>[4x]MNTIDAEVIIVGAGPTGLMLAGELRLNNVSTIVLDRLAEPMQQSRALGFSARTIEEFDQRGL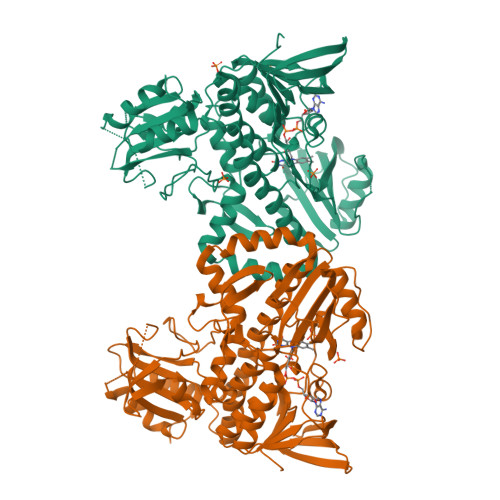LARFGEVGTIPFGHFGGVPLDYRVIKGGSYGARGIPQSRTEGMLAAAAVELGAELRRGQEVVSIDDDGTGVAVVVRTADGEQTLRAKYLVGADGARSTVRKAAGIDFPGTDPTMEMWLADVAGCDLRLRFSGELVPGGMVMVLPLGPVAQRVVVFEHATGLRNSTEPPTFAEVADAFERLTGEDIRGGKPLWVSWFTDSSRQAAEYRRGRILLAGDAAHIHMPIGGQGMSAGIQDAVNLGWKLAAEIHGHAPEGLLDTYHTERHPVDGRVVMNTLAQRWLYLGGEAMQPLRELLGELVRYPDVQEHLVGMVTGLDIRYDVGAGEHPLLGRRIPNQELVGEFDGSGKSTTFEQLHRGRGVLFAFGDDTAGPQAATGWTDRVDVVRATPHTADPDDPFHGLDAVLVRPDGYVAWVAPAGAGAAGLDEALSRWFGPSR> GAQVSAQKSGTHETGNIA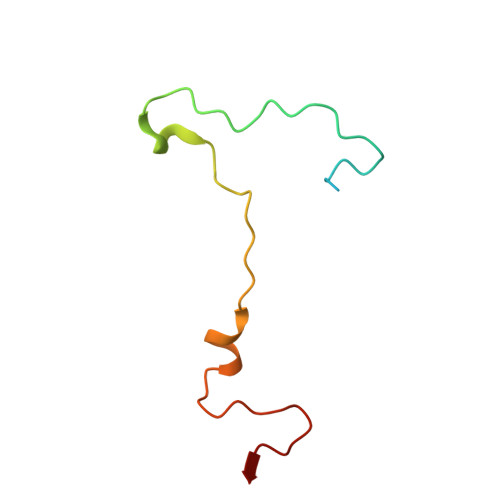TEGSTINFTNINYYKDSYAASASRQDFTQDPTKFTSPVLDAIKEAAAPLQ>MSEQYSEINTDTLERVTEIFKALGDYNRIRIMELLSVSEASVGHISHQLNLSQSNVSHQLKLLKSVHLVKAKRQGQSMIYSLDDIHVATM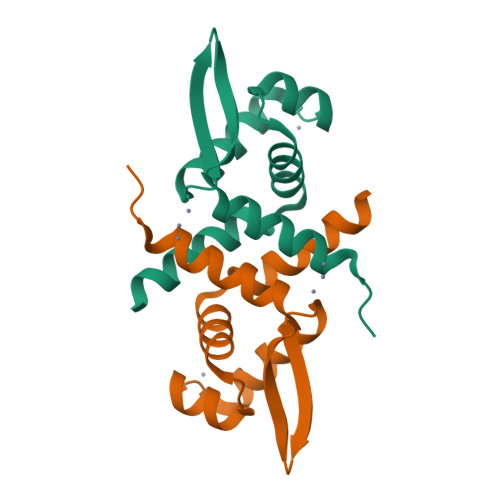LKQAIHHANHPKESGL[2x]>QQRRFPDDFLFGTATASYQIEGAWDEDGKGENIWDYMVHNTPEVIRDLSNGDIAADSYHNYKRDVEMMRELGLDAYRFSLSWARILPTGMANEVNPAGIAFYNNYIDEMLKYNITPLITLYHWDLPQKLQELGGFANPLISDWFEDYARVVFENFGDRVKMFITFNEPREICFEGYGSATKAPILNATAMGAYLCAKNLVTAHAKAYYLYDREFRPVQGGQCGITISVNWFGPATPTPEDEMAAELRRQGEWGIYAHPIFSAEGGFPKELSDKIAEKSAQQGYPWSRLPEFTEEEKAFVRGTSDFFGVNHYTAFLVSATERKGPYPVPSLLDDVDTGSWADDSWLKSASAWLTLAPNSIHTALTHLNNLYNKPVFYITENGWSTD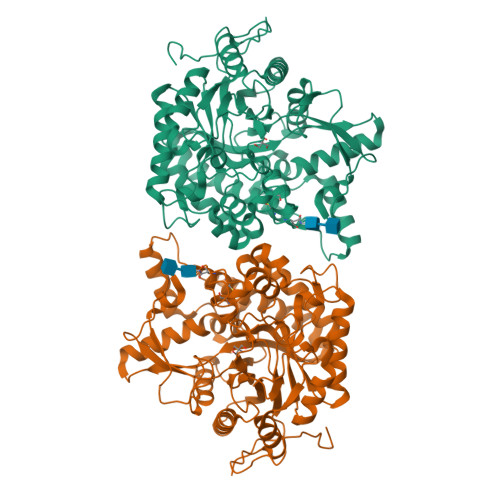ESRENSLIDDDRIQYYRASMESLLNCLDDGINLKGYMAWSLMDNFEWMEGYIERFGLYEVDFSDPARTRTPRKAAFVYKHIIKHRVVDYEYEPETMVMTIDEGH[6x]> AYQLYRNTTLGNSLQESLDELIQSQQITPQLALQVLLQFDKAINAALAQRVRNRVNFRGSLNTYRFCDNVWTFVLNDVEVREVTELIKVDKVKIVACDGKNTANSANTNTVPKLYRSVIEDVINDVRDIFLDDGVDEQVLMELKTLWENKLMQSRAVDGELFDTENVVVCQYDKIHRSKNK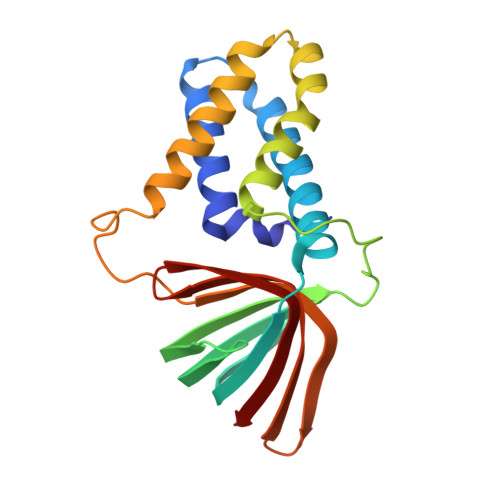WKFHLKDGIMNLNGRDYIFSKAIGDAEW> MDEKKLFLKALKKKFEGEDPDEKYTNFYCFGGWEQSARKKEFTEYAKKAAEKRGGIPFYNPDIGVPLGQRKLMAYRVSGTDAYVEGDDLHFVNNAAIQQMVDDIKRTVIVGMDTAHAVLEKRLGVEVTPETINEYMEAINHALPGGAVVQEHMVEVHPGLVEDCYAKIFTGDDNLADELDKRILIDINKEFPEEQAEQLKSYIGNRTYQVNRVPTIVVRTCDGGTVSRWSAMQIGMSFISAYKLCAGEAAIADFSYAAKHADVIEMGTIMPARRARGPNEPGGVAFGTFADIVQTSRVSDDPANVSLEVIAGAAALYDQVWLGSYMSGGVGFTQYAT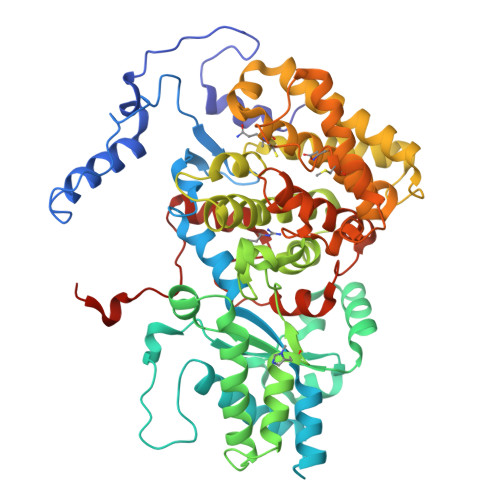AAYTDDILDDFVYYGMEYVDDKYGICGTKPTMDVVRDISTEVTLYSLEQYEEYPTLLEDHFGGSQRAAVAAAAAGCSTAFATGNSNAGINGWYLSQILHKEAHSRLGFYGYDLQDQCGASNSLSIRSDEGLIHELRGPNYPNYAMNVGHQPEYAGIAQAPHAARGDAFCTNPLIKVAFADKDLAFDFTSPRKSIAAGALREFMPEGERDLIIPAGK>[2x]QSNMKQEQMRLANQLCFSAYNVSRLFAQFYEKKLKQFGITYSQYLVLLTLWEENPQTLNSIGRHLDLSSNTLTPMLKRLEQSGWVKRERQQSDKRQ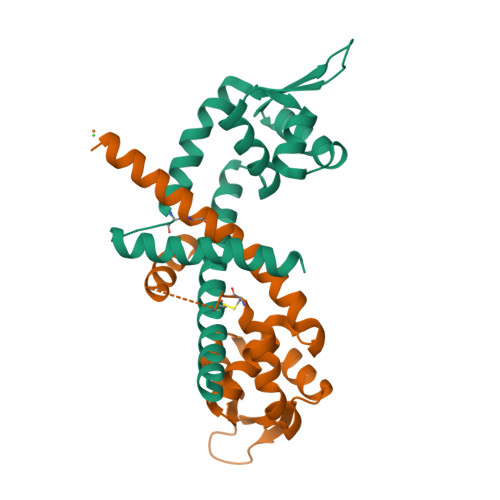LIITLTDNGQQQQEAVFEAISSCLPQEFDTTEYDETKYVFEELEQTLKHLIEK>MIKAVVFDAYGTLFDVQSVADATERAYPGRGEYITQVWRQKQLEYSWL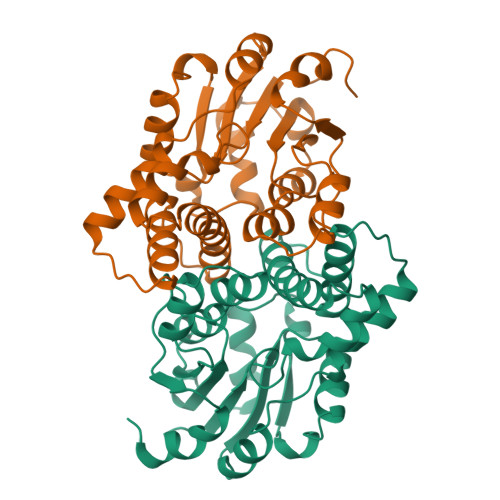RALMGRYADFWGVTREALAYTLGTLGLEPDESFLADMAQAYNRLTPYPDAAQCLAELAPLKRAILSNGAPDMLQALVANAGLTDSFDAVISVDAKRVFKPHPDSYALVEEVLGVTPAEVLFVSSNGFDVGGAKNFGFSVARVARLSQEALARELVSGTIAPLTMFKALRMREETYAEAPDFVVPALGDLPRLVRGMAGAHLAPAV[2x]> EARRTRKYLELYIVADHTLFLTRHRNLQHTKQRLLEVANYVDQLLRTLDIQVALTGLEVWTERDRSRVTQDANATLWAFLQWRRGLWAQRPHDSAQLLTGRAFQGATVGLAPVEGMCRAESSGGVSTDHS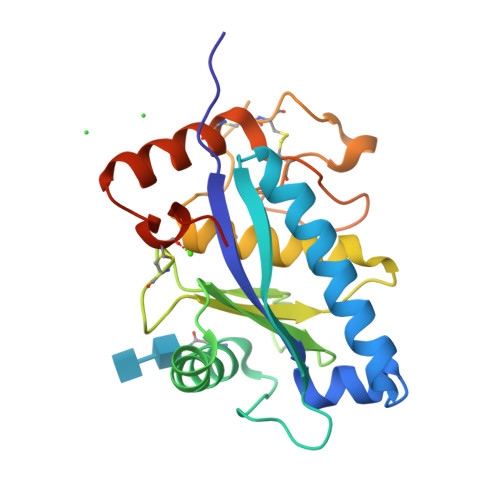ELPIGAAATMAHEIGHSLGLSHDPDGCCVEAAAESGGCVMAAATGHPFPRVFSACSRRQLRAFFRKGGGACLSNAPSGHHHHHH> MGSSHHHHHHSQDPMHKLAIIGYGAAGFAAMIKANELGVKPVLIGKGEIGGTCVNVGCVPSKRMLYIAEIYKKAREVTGSEVYPPFSSFQEKDGLVQEMRKTKYEDLLSYYDVELIQGEARFISPHAVKVNGQVIEAEKFVIATGSSP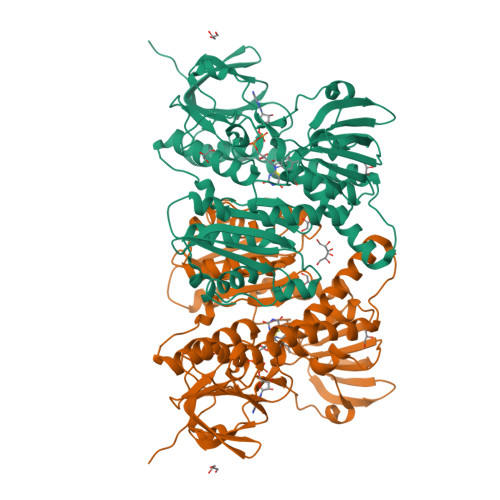LIPRIPGLDKVGFWTNREALSPDRRIDSLAVIGGRALALEFAQMYSRMKVEVAILQRSPVLIPDWEPEASVEARRIMENDGVAVVTGVNVKEVRKGAGKIVITDKGEVEADEILLATGRKPNVDLGLENAGVRLNERGGIKVDDELRTDNPHIYAAGDVLGGKMLEALAGRQGSIATENALTGSHKRVDENAVPQVIFTQPNLARVGLTEAEARAKEGEVEARVLPMSSVAKAEIINSRLGFVKMVTMNGRIVGVHAVGENVAEMIGEAALAIRFGATVHDLIDTVHMFPTIAESLRLVALAFRSDVSRLSCCV In this work we have determined the structure of SpvD, a S. typhimurium SPI-2 T3SS effector protein that inhibits the NF-κB signaling pathway. In this work we determined the structure of SpvD and showed that it is a hydrolase with a papain-like fold and a catalytic triad composed of Cys-73, His-162, and Asp-182. Structurally, SpvD can be classified as belonging to the CA clan of cysteine proteases that contains papain and related proteases (MEROPS peptidase database). Although SpvD is highly conserved among different serovars of S. enterica, serovars Typhimurium and Enteritidis differ in containing an arginine or glycine, respectively, at residue 161 near the active site.

Interestingly, conversion of the SpvD sequence to that of the Enteritidis strains increased the activity observed in the DUB-GloTM protease assay. To explain why the Gly-161 polymorphism leads to greater activity, we crystallized an inactive (C73A) form of the variant in the presence of RLRGG-AML substrate. Although density for the RLRGG-AML substrate was not observed, we were able to build additional loops (two of them near the active site) that were disordered in the previously obtained SpvD4CS/R161 structure. To map a potential ligand binding site on SpvD, we superimposed the catalytic triad with that of the UCH-L3 ubiquitin hydrolase crystallized in complex with ubiquitin. The position of the superimposed five C-terminal amino acids of ubiquitin (RLRGG) is unobstructed in the SpvD4CS/G161/C73A variant (right), whereas in SpvD4CS/R161, binding would be impeded by the side chain of Arg-161, which restricts access to the active site (left). Modeling of the RLRGG DUB-GloTM substrate onto the Arg-161 or Gly-161 structures provides a rationale for this observation, clearly showing that the side chain at position 161 forms part of the active site groove and that an arginine side chain here restricts access to the catalytic triad. When compared with the Typhimurium SpvDA154/R161 variant, SpvD with a single polymorphism (Gly-161) was more potent in (i) the DUB-GloTM protease assay, (ii) inhibition of the NF-κB luciferase assay in PMA-stimulated cells, and (iii) virulence in mice. Furthermore, we demonstrate that a natural SpvD polymorphism significantly affects virulence and NF-κB inhibition in PMA-stimulated cells, leading us to hypothesize that the substrate hydrolyzed by SpvDG161 might be part of a signaling pathway involving protein kinase C.

> GPGMRVSGSASSQDIISRINSKNINNNDSNEVKRIKDALSIESKERILYPQNLSRDNLKQMARYVNNTYVHYSGNAVLLSACLHYNIHHRQDILSSKNTASPTVGLDSAIVDKIIFGHELNQSYSLNSIDEVEKEILNRYDIKRESSFIISAENYIAPIIGESGHDFNAVVISEYDKKPYVQFIDSWKTSNILPSLQEIKKHFSSSGEFYVRAYDEKHD>EIPLKYGATNEGKRQDPAMQKFRDNRLGAFIHWGLYAIPGGEWNGKVYGGAAEWLKSWAKVPADEWLKLMDQWNPTKFDAKKWAKMAKEMGTKYVKITTKHHEGFCLWPSKYTKYTVANTPYKRDILGELVKAY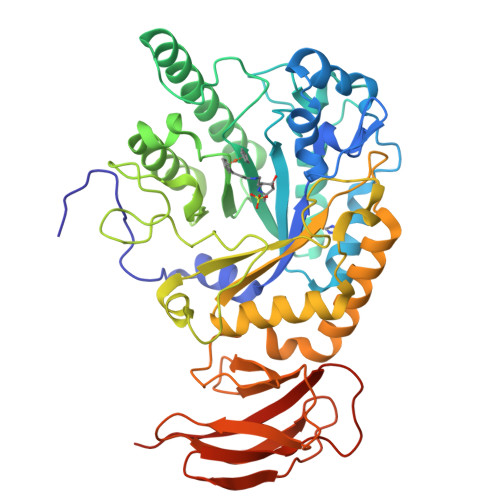NDEGIDVHFYFSVMDWSNPDYRYDIKSKEDSIAFSRFLEFTDNQLKELATRYPTVKDFWFDGTWDASVKKNGWWTAHAEQMLKELVPGVAINSRLRADDKGKRHFDSNGRLMGDYESGYERRLPDPVKDLKVTQWDWEACMTIPENQWGYHKDWSLSYVKTPIEVIDRIVHAVSMGGNMVVNFGPQADGDFRPEEKAMATAIGKWMNRYGKAVYACDYAGFEKQDWGYYTRGKNDEVYMVVFNQPYSERLIVKTPKGITVEKATLLTTGEDITVVETTRNEYNVSVPKKNPGEPYVIQLKVRAAKGTKSIYRDALT[4x]>MNNSEDPFQQVVKDTKEQLNRINNYITRHNTAGDDDQEEEIQDILKDVEETIVDLDRSIIVMKRDENEDV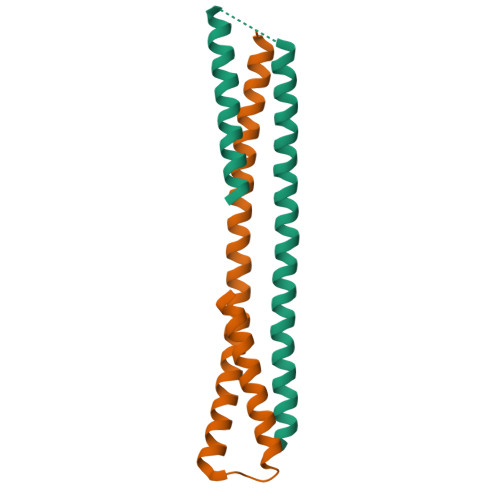SGREAQVKNIKQQLDALKLRFDRRI[2x]>MVEKPYDYVFFENSLMKGDYFYSQAKYTSPSWIKNARHHLPVAGSVAFTPGNSLELTYVSAPGGDWYSEIQYCPVRGNDFFREPSTLSMQVRLRESMNAAALPNIAIRYADSTYTQYLNLRNYLKDTRPGVWHPVSIPLEDFGLNAVNDTNIKKLAAVALRPGTADGNEYTIYLDDIELLPASLPSVSALNAPVLQEAKAYERHIDIKWIPQSKEDIKYYRIYRSFDGITYQPVAVR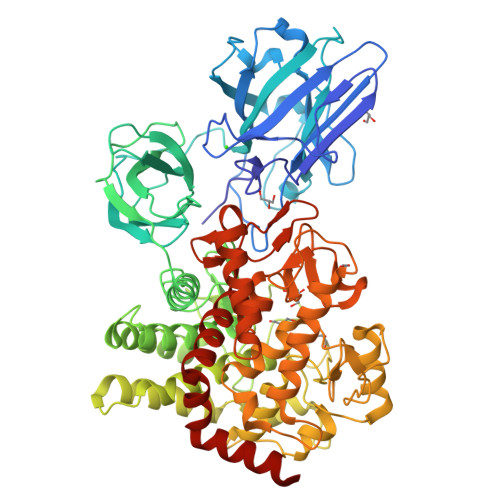RPWMNRYTDFLGEVGKKAYYKVTAVDYALNESNDSQTVSATTYPMTDEQLLDMVQEANFRYYWEGAEPNSGLARENIPGRNDMIATGASGFGIMAIVAGIERGFITREEGVQRFLKITSFLEKADKFHGAVSHFIDGTTGKTVAFFGPKDNGGDLVETSFLFQGLLTARQYFNQENDKEKQIRKSIDNLWKNVEWSWYKQFKDSPYLYWHWSPDQAWVINHKLIGWNETMITYMLAIMGPKYGISPEMYYSGWASQEEYAQEYRADWGRVEDGKMYTNGNTYYGENLKVGVSNGGPLFFIHYSYLGLDPHKFTDKYTNYFENNQKMAKINQRYCIENQGGYVGYGEDCWGLTASDFAWNYQAQEPMPHRDNGTMAPTGALASFPYTPDASMKALRNYYRNHGSFLWGEYGFRDAFNLTVNWVSPLFMGLNQAPVTVMIENYRTNLLWNLFMSHPDVQKGIQKIQSIKLEHHHHHH[2x]> MKLLWQVTVHHHTWNAILLPFVYLTAQVWILCAAIAAAASAGPQNCPSVCSCSNQFSKVVCTRRGLSEVPQGIPSNTRYLNLMENNIQMIQADTFRHLHHLEVLQLGRNSIRQIEVGAFNGLASLNTLELFDNWLTVIPSGAFEYLSKLRELWLRNNPIESIPSYAFNRVPSLMRLDLGELKKLEYISEGAFEGLFNLKYLNLGMCNIKDMPNLTPLVGLEELEMSGNHFPEIRPGSFHGLSSLKKLWVMNSQVSLIERNAFDGLASLVELNLAHNNLSSLPHDLFTPLRYLVELHLHHNPWNCDCDILWLAWWLREYIPTNSTCCGRCHAPMHMRGRYLVEVDQASFQCSAPFIMDAPRDLNISEGRMAELKCRTPPMSSVKWLLPNGTVLSHASRHPRISVLNDGTLNFSHVLLSDTGVYTCMVTNVAGNSNASAYLNVSTAGTHHHHHH;> MLHLLALFLHCLPLASGDYDICKSWVTTDE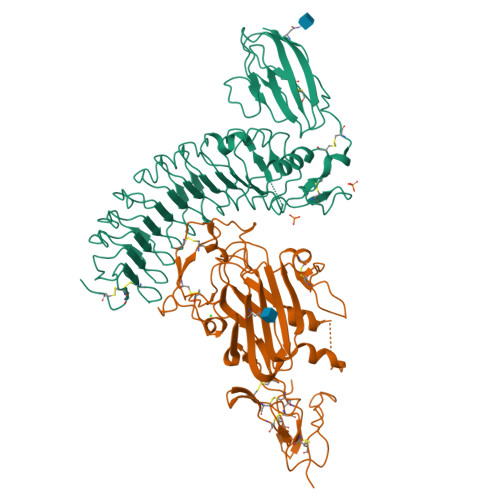GPTWEFYACQPKVMRLKDYVKVKVEPSGITCGDPPERFCSHENPYLCSNECDASNPDLAHPPRLMFDKEEEGLATYWQSITWSRYPSPLEANITLSWNKTVELTDDVVMTFEYGRPTVMVLEKSLDNGRTWQPYQFYAEDCMEAFGMSARRARDMSSSSAHRVLCTEEYSRWAGSKKEKHVRFEVRDRFAIFAGPDLRNMDNLYTRLESAKGLKEFFTLTDLRMRLLRPALGGTYVQRENLYKYFYAISNIEVIGRCKCNLHANLCSMREGSLQCECEHNTTGPDCGKCKKNFRTRSWRAGSYLPLPHGSPNACAGTHHHHHH> MASAELAKPLTLDQLQQQNGKAIDTRPSAFYNGWPQTLNGPSGHELAALNLSASWLDKMSTEQLNAWIKQHNLKTDAPVALYGNDKDVDAVKTRLQKAGLTHISILSDALSEPSRLQKLPHFEQLVYPQWLHDLQQGKEVTAKPAGDWKVI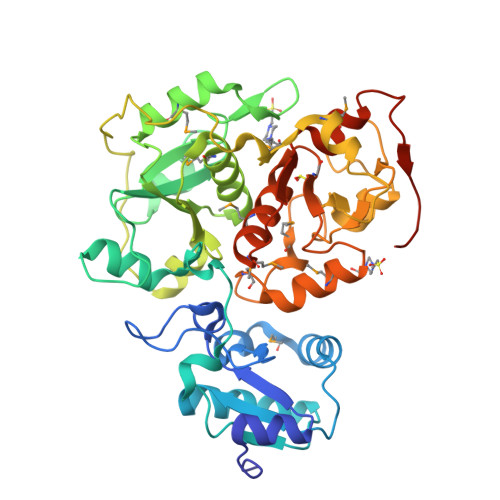EAAWGAPKLYLISHIPGADYIDTNEVESEPLWNKVSDEQLKAMLAKHGIRHDTTVILYGRDVYAAARVAQIMLYAGVKDVRLLDGGWQTWSDAGLPVERGTPPKVKAEPDFGVKIPAQPQLMLDMEQARGLLHRQDASLVSIRSWPEFIGTTSGYSYIKPKGEIAGARWGHAGSDSTHMEDFHNPDGTMRSADDITAMWKAWNIKPEQQVSFYCGTGWRASETFMYARAMGWKNVSVYDGGWYEWSSDPKNPVATGERGPDSSKLEHHHHHH Homologues of the 90-residue ReoM protein are found across the entire Firmicute phylum, and include IreB, a substrate of the protein serine/threonine kinase IreK and its cognate phosphatase IreP from Enterococcus faecalis, whereas ReoY homologues are present only in the Bacilli. Therefore, ReoM, ReoY and MurZ likely affect the ClpCP-dependent degradation of MurA. PrkA phosphorylates ReoM on Thr7 and PrpC reverses this reaction in vitro; ReoM phosphorylation at Thr7 in vivo has also been observed by phosphoproteomics. Our data are consistent with a model in which PrkA-phosphorylated ReoM no longer activates ClpCP, which leads to MurA stabilisation and the activation of PG biosynthesis.

Purified ReoM yielded crystals that diffracted to a maximum resolution of 1.6 Å. Other than IreB, there are no structural homologues of ReoM with functional significance in the PDB. The helical bundles in both ReoM and IreB associate into homodimers with α-helices two and four from each protomer forming the majority of the homodimer interface, and these residues are highlighted in Figure 6B. In agreement with the IreB structural analysis, 1200 Å2 of surface area is buried in the ReoM dimer interface, representing 9% of the total solvent accessible surface area. Other than the compact helical bundle of ReoM, there is a ~ 16 residue-long N-terminal tail, with B-factors 25% higher than the rest of the protein, prior to the start of α-helix one at residue Ile17. Consequently, it is possible to visualise Thr7, the target for phosphorylation by PrkA, in the flexible N-terminal region in both chains. The side chain of Thr7 in both chains makes no intramolecular interactions and is thus amenable to phosphorylation by PrkA. Alternatively, the presence of a sulphate ion (a component of the crystallisation reagent) adjacent to the sidechain of Thr7 could mimic what P-ReoM might look like. The sulphate ion is captured by a positively-charged micro-environment from a symmetry-equivalent molecule. ReoM could thus react to phosphorylation by a substantial movement of Thr7 to interact with this positively-charged surface, which comprises arginines with levels of conservation (Arg57 [57% conserved], Arg62 [99%], Arg66 [76%], Arg70 [98%]) amongst all 2909 ReoM homologues present at NCBI approaching that of Thr7 (96%).

>[2x]MDSKDQTMFYNFGDDSIEEDVKKLMKQVYVALEEKGYNPVNQIVGYLLSGDPAYIPRHKDARSMIRRLERDEIIEELVKAYLKNNEIGEK> ELPNIMHPVAKLSTALAAALMLSGCMPGEIRPTIGQQMETGDQRFGDLVFRQLAPNVWQHTSYLDMPGFGAVASNGLIVRDGGRVLVVDTAWTDDQTAQILNWIKQEINLPVALAVVTHAHQDKMGGMDALHAAGIATYANALSNQLAPQEGLVAAQHSLTFAANGWVEPATAPNFGPLKVFYPGPGHTSDNITVGIDGTDIAFGGCLIKDSKAKSLGNLGDADTEHYAASARAFGAAFPKASMIVMSHSAPDSRAAITHTARMADKLR

The bacterial metallo-β-lactamases (MBLs) catalyze the inactivation of β-lactam antibiotics. Class B members, known as the metallo-β-lactamases (MBLs), are structurally distinct from the Class A, C, and D enzymes, require one or two zinc ions for catalytic activity, and are not inhibited by currently approved therapeutics. One variant of significance is NDM-4, first identified in 2012 (17). Although it differs from NDM-1 by a single amino acid substitution, namely M154L, it demonstrates increased enzymatic activity against the carbapenems and several cephalosporins.

The first crystals of NDM-4 utilized in this investigation were grown at room temperature using poly(ethylene glycol) 3350 as the precipitant (pH 6.0). They belonged to the space group P21 with a monomer in the asymmetric unit. The model of the enzyme was refined to an overall R-factor of 17.9% at 1.3 Å resolution. The electron density for the polypeptide chain was continuous from Gly 42 to Arg 270. The two zincs that form the binuclear metal center are separated by 3.5 Å. Zn1 is ligated by the side chains of His 120, His 122, His 189 at the so-called “histidine” site and a bridging water (or hydroxide ion) in a distorted tetrahedral arrangement. The bond lengths between Zn1 and the imidazole nitrogens of His 120, His 122, and His 189 are 2.0, 2.1, and 2.0 Å, respectively, whereas the distance between Zn1 and the bridging water is 1.8 Å. Zn2 is surrounded in an octahedral coordination sphere provided by the side chains of Asp 124, Cys 208, His 250 at the so-called “cysteine” site, the bridging solvent and two water molecules. The metal-ligand distances are all ∼2 Å with the exception of that formed between the zinc ion and the thiolate of Cys 208, which is 2.5 Å.> AATTGYDAVDDLLHYHERGNGIQINGKDSFSNEQAGLFITRENQTWNGYKVFGQPVKLTFSFPDYKFSSTNVAGDTGLSKFSAEQQQQAKLSLQSWADVA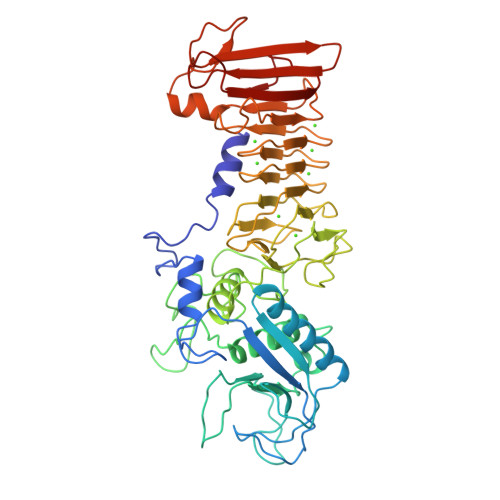NITFTEVAAGQKANITFGNYSQDRPGHYDYGTQAYAFLPNTIWQGQDLGGQTWYNVNQSNVKHPATEDYGRQTFTHEIGHALGLSHPGDYNAGEGNPTYRDVTYAEDTRQFSLMSYWSETNTGGDNGGHYAAAPLLDDIAAIQHLYGANLSTRTGDTVYGFNSNTGRDFLSTTSNSQKVIFAAWDAGGNDTFDFSGYTANQRINLNEKSFSDVGGLKGNVSIAAGVTIENAIGGSGNDVIVGNAANNVLKGGAGNDVLFGGGGADELWGGAGKDIFVFSAASDSAPGASDWIRDFQKGIDKIDLSFFNKEAQSSDFIHFVDHFSGAAGEALLSYNASNNVTDLSVNIGGHQAPDFLVKIVGQVDVATDFIV> MFKTEFEFPEELKTKLQEHINYFPKKRQAILLCLHEIQNYYGYIPPESLKPLADMLELPLNHVEGVVAFYDMFD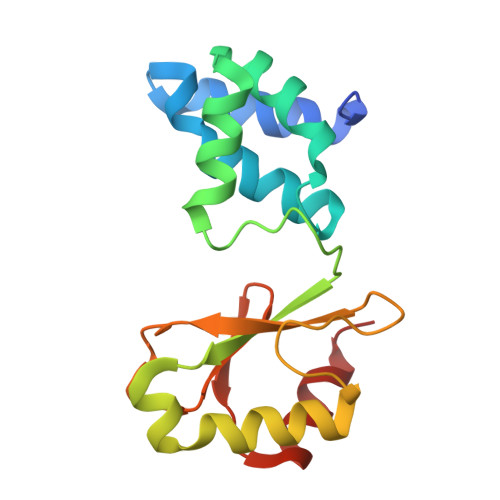REDKAKYRIRVCVSIVCHLMGTNKLLKALENILGIKPGEVTPDGKFKIVPVQCLGACSEAPVFMVNDDEYKFESEVQLNEILSRYT>MVRPSFSSIVEVKIGGAKLPDTIAPMLTDGWVDQGVNVPAAFRLTFRDPYHRLLGDLNVQFGTKVVITPIADGQGKNNPLLTGEVTGLETDYDGTGSFTVIRGYDYGHRLMRQRRVAAYRNQKASDIARKLVQMDGVSVGRIQPTKGTYAFIAQPNVTDWDFLARLADENKMIMYLDSKGKFRFVTPKPSAGAPSPNTDGDQSAFVLQAGHDILRLRAAVTAADQIGKVESRGWNVTTKKKITEIAPATTDPGISIKWTPGTAAGKFKPGKLVETANPYDKQDEVQNAAKALASDVTASFSELEVAANGHPDLRPGVPVALSDVGTPFEGKYTVTSVRHHFGDGVAYESWITVSGRQWRSLYGLASGGGGSDPASATRLPSVANAIVTDVQDPLKQGRVKLQFPWLDDTYVSDWARSVQMGGVAGGGIFPMDVGDEVLVAFDRGALDHPFVIGGLYNGRDVPTKSDVPLHDGLKKKAVRHTLSDRQGNRVDLLSQRTGGRKQGVRIASGNDKLTINLDRTKTEITVDSKGSVSITGSRSVSVDAGTDLSLSARRSLTIKSGGPLSIQGGSTINMRSGGLVGVNAGGALNLGAGGA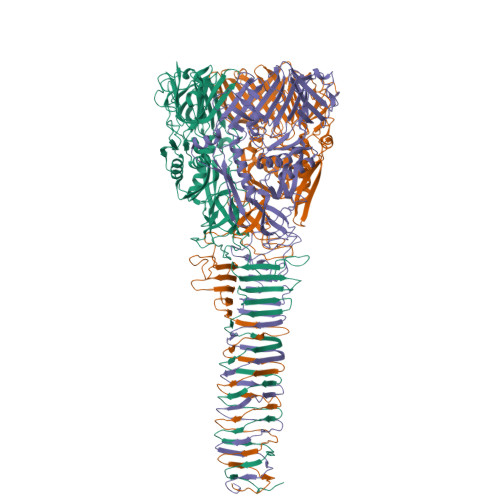ATLSAGAATTISGTVNVQINSVMTRVIGATFEVKTPIFKVATIPVPGL[3x]E. coli aspartate aminotransferase (AAT) is a pyridoxal phosphate (PLP)-dependent enzyme that catalyses the reversible transamination of l-aspartate with α-ketoglutarate, yielding oxaloacetate and l-glutamate. During its catalytic cycle, AAT undergoes hinge movement to switch between an open conformation, in the ligand-free form, and a closed conformation upon association with substrates or inhibitors. Using our approach, we enrich the less populated but catalytically active closed conformation in order to increase catalytic efficiency (kcat/KM) with the non-native substrate l-phenylalanine, leading to altered substrate selectivity. Steady-state kinetics reveal kcat/KM increases of up to 100-fold towards this aromatic amino acid, resulting in a selectivity switch of up to 1900-fold, and structural analyses by room-temperature X-ray crystallography and multitemperature nuclear magnetic resonance (NMR) spectroscopy confirm that the conformational landscape is remodeled to favor the target state.

To determine if these differences in the temperature dependence of exchange could be observed in the crystal state, we also solved the maleate-free structures of WT, HEX, and VFIT at 303 K, and calculated isomorphous difference density maps by subtracting electron density at 278 K. By contrast, similar comparisons for WT and HEX showed relatively little difference density. Upon soaking crystals of the WT enzyme to remove the bound inhibitor, we observed that one subunit (chain A) within the enzyme homodimer was in the open conformation, confirming that the soaking procedure was able to remove the bound maleate, and that the crystal lattice could accommodate the domain rotation required for opening and closing of this subunit. The 19F spectrum of WT at 278 K showed a single peak centered at approximately ‒60 ppm that shifts downfield as temperature is increased, similar to what is observed for free 4-trifluoromethyl-l-phenylalanine in solution.

>MAHHHHHHVGTFENITAAPADPILGLADLFRADERPGKINLGIGVYKDETGKTPVLTSVKKAEQYLLENETTKNYLGIDGIPEFGRCTQELLFGKGSALINDKRARTAQTPGGTGALRVAADFLAKNTSVKRVWVSNPSWPNHKSVFNSAGLEVREYAYYDAENHTLDFDALINSLNEAQAGDVVLFHGCCHNPTGIDPTLEQWQTLAQLSVEKGWLPLFDFAYQGFARGLEEDAEGLRAFAAMHKELIVASSYSKNFGLYNERVGACTLVAADSETVDRAFSQMKAAIRANYSNPPAHGASVVATILSNDALRAIWEQELTDMRQRIQRMRQLFVNTLQEKGANRDFSFIIKQNGMFSFSGLTKEQVLRLREEFGVYAVASGRVNVAGMTPDNMAPLCEAIVAVL[2x]> LASF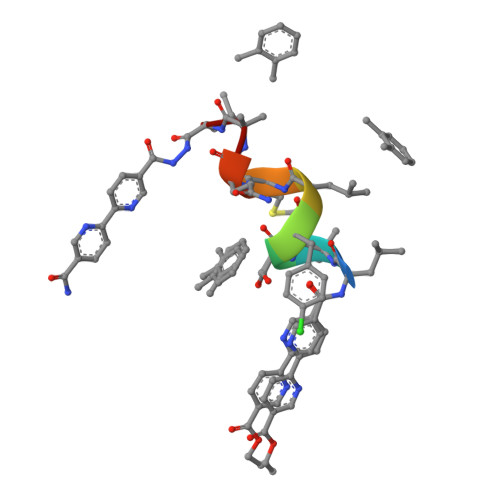LMQAL> MHKEVKARYDEQMVLKKAALLYHFQPEQVTFLADAENYVYEYTDEKGSSYILKITHTIRRSSTYILGEMDWIRYLSQHGISVAKPVLSARGKDVEAIPDQAGGAFLLRVYEKAPGRKVTEADWNGQLFQALGAYTGRMHQTTKQYQVKDPRYKRQEWYEEEQLKLETYIPSDQTVVLQRKDELMQKLHQLRISKDVYGLVHADLHHGNFHYHQGEIIAFDFDDCGYHWFINDISILLYNVLWYPVIPYEDKAE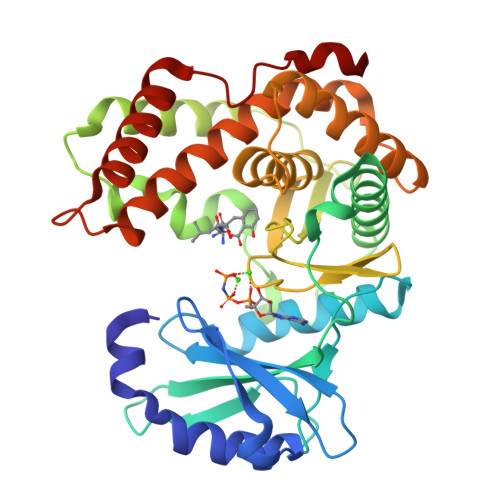FTGEFMSHFLKGYRQENELDDAWLATIPDFLMLRHMLIYGLLHQAFDLRTLSADESAMLARFRKEIEDKTPITPFDFHQLTT>[12x]MSMQQETSHMTAAPQTNGHQIFPEIDMSAGDSSSIVRATVVQASTVFYDTPATLDKAERLLSEAAENGSQLVV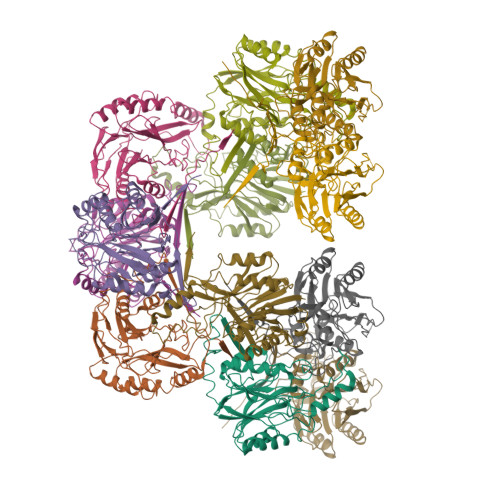FPEAFIGGYPRGSTFELAIGSRTAKGRDDFRKYHASAIDVPGPEVERLALMAKKYKVYLVMGVIEREGYTLYCTVLFFDSQGLFLGKHRKLMPTALERCIWGFGDGSTIPVFDTPIGKIGAAICWENRMPSLRTAMYAKGIEIYCAPTADSRETWLASMTHIALEGGCFVLSANQFCRRKDYPSPPEYMFSGSEESLTPDSVVCAGGSSIISPLGIVLAGPNYRGEALITADLDLGDIARAKFDFDVVGHYSRPEVFSLNIREHPRKAVSFKTSKVMEDESVHHHHHH>[4x]MARLDDLFIIHDTYVCLLSDHLLPNVIPVIQAPPQRVILLYTPNNKERVQRFRQATESVPTEIIEKQVHPYQYAQTQRICDEILEQFPNAILNVTGGTKIMALAAFDRFRHNHRPIIYVDSDSQRILYLHNGESERLGDPLTVKQYLACYGFKADNINRQDNLPKTWREVEDLFAQNSTKWQNQLGRLNWIAAQQQPIFTLQTGELQDLLLKANLIKPAEAKNAGFQFTSDQARQFINGGWFEHYVYSLLRQISAQYPIKNLTKNIEISNDSVSNELDVVFLYHNKLHVIECKTRHFTADGKINPMETIYKIDSVTNRVAGIKGKSMFASYYPLTQAAKKRCLNNSIYVSDQPSQLHHQLIKWINA

Type III CRISPR systems detect foreign RNA and typically generate cyclic oligoadenylate (cOA) second messengers that bind to ancillary proteins with CARF (CRISPR associated Rossman fold) domains. Here we show that Can2, a widely distributed CARF-superfamily protein associated with type III CRISPR systems, is a cA4-activated DNA nickase and RNase that can provide immunity against bacteriophage in vivo. Can2 has two distinct domains, linked by a 15-residue highly flexible loop. At the N-terminus there is a CARF domain (residues 3–151) and at the C-terminus a nuclease domain (residues 166–366).

SthCan2, with selenomethionine incorporated for phasing, was co-crystallised with cA4. There are four protein molecules in the asymmetric unit, which form two dimers each bound to a molecule of cA4. Unambiguous electron density in the Fobs – Fcalc map at 3σ at the interface between the CARF domains in the dimer of Can2 corresponded to a molecule of cA4 enclosed in the binding site. The cA4 molecule makes symmetrical interactions with each Can2 monomer, which differs from the asymmetric interactions made between Can1 and cA4. All interactions made between Can2 and cA4 are solely from the CARF domains. Hydrogen bonds form between cA4 and main chain residues of Asp20, His21, and Lys99 and side chain residues of Ser19, Asp20, Thr42, Lys99, Tyr118 and Ser121 in both molecules of the Can2 dimer. The structure of Can2 bound to cA4 represents the active state of the enzyme. The dsDNA substrate from EndoMS in the superimposed structures sits in the cleft between the two Can2 nuclease domains. There appears to be room in this cleft to accommodate canonical dsDNA if it is assumed that the flexible loop (Thr294–Asn304) can move to accommodate the DNA, allowing nicking by Can2. Clearly ssRNA as a smaller molecule could also be accommodated in this cleft. This analysis suggests that the mechanism of cA4-dependent activation is likely to be via allosteric structural reorganisation that opens the cleft, allowing access to DNA and RNA substrates.>GSRGSNTIGARLNRVEDKVTQMDQRMALITD[3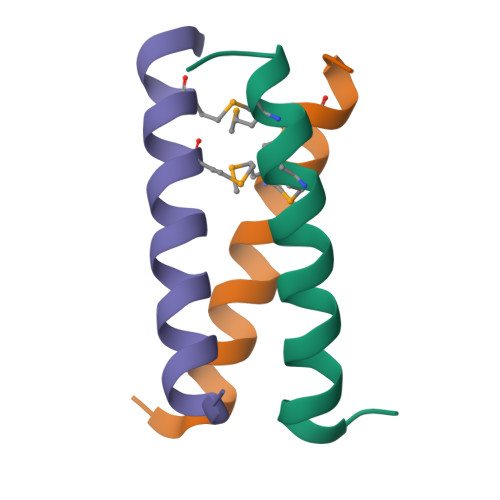x]> QV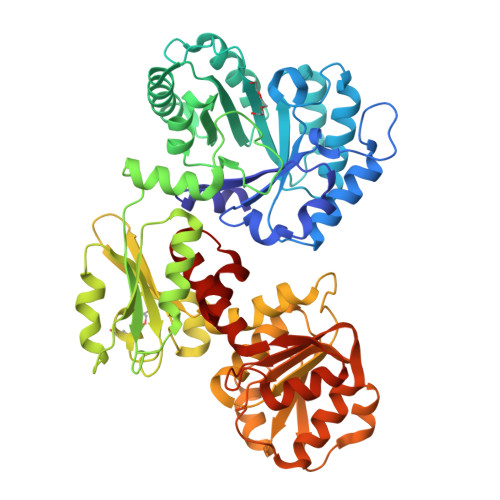LQKFKTKKRSTFLTLNYPRIEDALPTLRDVTVGCDAIEVRVDYLKDPKSSNGISSLDFVAEQISLLRCSTTLPIIFTIRTISQGGLFPNDKEEEAKELMLSAMRYGCDFVDVELGWSSETINILYQHKGYTKLIMSWHDLSGTWSWARPHEWMQKVELASSYADVIKLVGMANNLNDNLELEEFRTRITNSMDIPLILFNMGRFGQLSRILNKFMTPVTHPLLPSKAAPGQLTVKQLNEARVLIGEILPEKFFLFGKPIKHSRSPILHSTAYELLGLPHTYEAFETDTVDEVQKVLNLPDFGGANVTIPYKLSVMKFMDELSDEARFFGAVNTIIPIRIGDKLVLRGDNTDWRGIYDTFANALDGVSLRDTNGLVIGAGGTSRAAIYSLHRLGVSRIYLLNRTLANSYRVQDVFPPDYNIHIIDSDNIPSEELSSVTLSAVVSTIPADIELPEKVASVIKALLANKADGGVFLDMAYKPLHTPLMAVASDLEWKCCNGLEALVRQGLASFHLWTGMTAPFDAVYQKVIE>AQPDIKFASKEYGVTIGESRIIYPLDAAGVMVSVKNTQDYPVLIQSRIYDENKEKESEDPFVVTPPLFRLDAKQQNSLRIAQAGGVFPRDKESLKWLCVKGIPPKDEDIWVDDATNKQKFNPDKDVGVFVQFAINNCIKLLVRPNELKGTPIQFAENLSWKVDGGKLIAENPSPFYMNIGELTFGGKSIPSHYIPPKSTWAFDLPKGLAGARNVSWRIINDQGGLDRLYSKNVTL[2x];>[4x]ADLTASFTATATLVEPARITLTYKEGAPITIMDNGNIDTELLVGTLTLGGYKTGTTSTSVNFTDAAGDPMY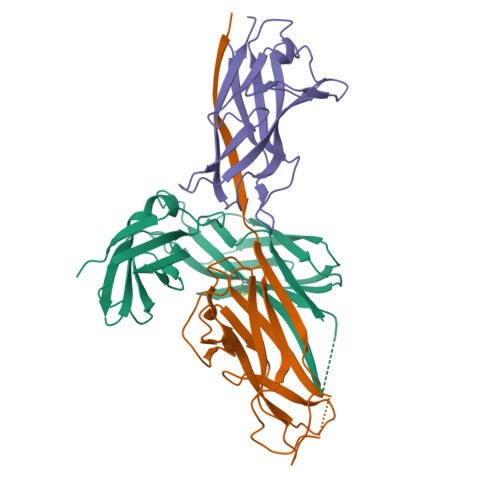LTFTSQDGNNHQFTTKVIGKDSRDFDISPKVNGENLVGDDVVLATGSQDFFVRSIGSKGGKLAAGKYTDAVTVTVSNQ> MGSSHHHHHHSQDPNSLVPRGSPQVAEFVSEMTRDYGFAGEQLMGLFRDVNRKQSILDAI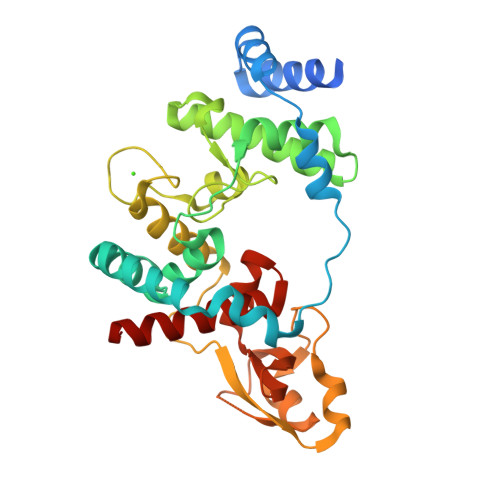SRPAERVKQWKEYRPIFISDARISRGVDFWNKHAEDLARAEKEYGVPAEIIVSIIGVETFFGRNTGSYRVMDALSTLGFDYPPRADFFRKELREFLLLAREQQVDPLSLTGSYAGAMGLPQFMPSSFRAYAVDFDGDGHINIWSDPTDAIGSVASYFKQHGWVTGEPVVSVAEINDESAESAVTRGVDPTMSLGELRARGWRTHDALRDDQKVTAMRFVGDKGIEYWVGLPNFYVITRYNRSAMYAMAVYQLAGEIARARGAH>[2x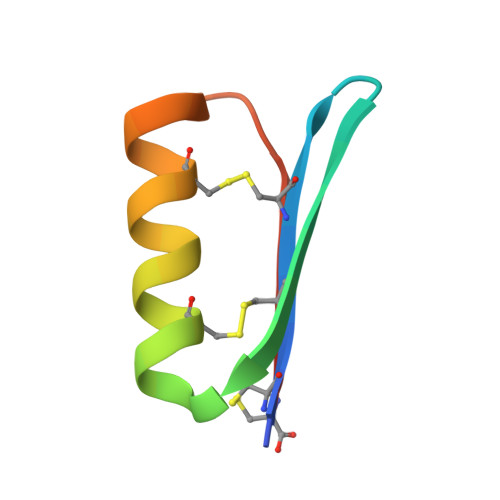]GSCFCVCITGPQWDYRYGNKEQCKKFLTECEQKNPGAEVEIQC>[2x]HMASQKVKEPTVSNADWSKPYRPFRIAGNLYYIGTYDLACYLITTKQGNIIVNTGLAASALQIKNNIKALGFKLTDTKILLTTQAHYDHLGAMAEIKKITGAKLMADEGDATVMADGGSSDYAFGGHGSMFEPIIADRLLHDKDTIQLGDTKLVMLHHPGHTKGSCSFLFDTKDEQR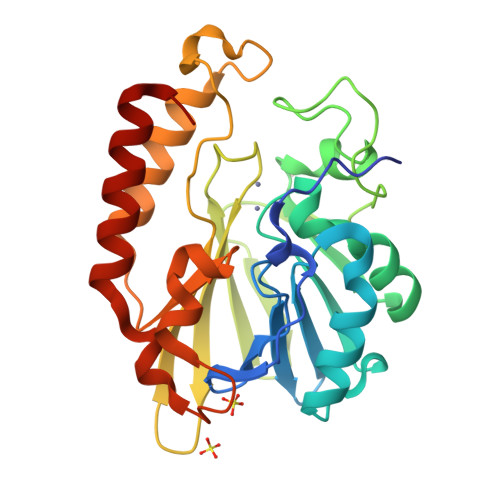SYRILIANMPTIVIEKKFSEVSSYPGIAKDYAYTLQAMKNLSFDIWVASHASQFSMHSKHKPGDGYNPKSFMDRKGYDESLDKLQKEYEKHLNEN> GGGRGKLEDVEAEKKLWESDDAWELRKAFMLAHYDDYPKIQLQCLSQLFINV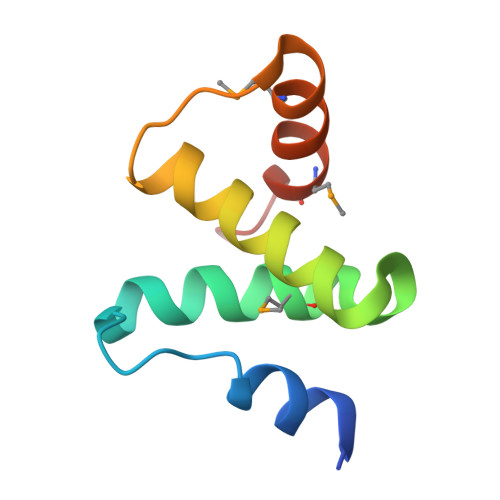TLLGCEYSQTLMQKIRTMGAGIAANK>GLESFSLTSHEKKFGVNIEFSDVNFSYPKQTNHRTLKSINFFIPSGTTCALVGHTGSGKSTIAKLLYRFYDAEGDIKIGGKNVNKYNRNSIRSIIGIVPQDTILFNETIKYNILYGKL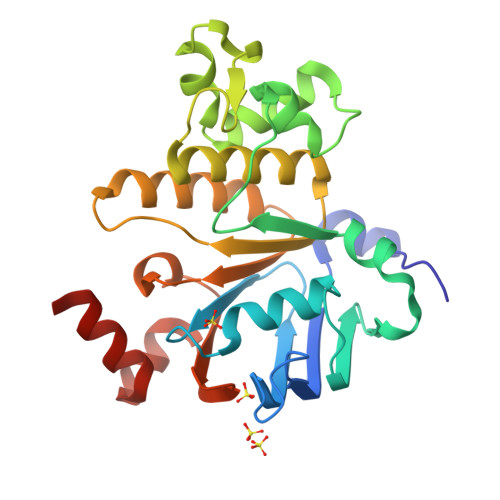DATDEEVIKATKSAQLYDFIEALPKKWDTIVGNKGMKLSGGERQRIAIARCLLKDPKIVIFDEATSSLDSKTEYLFQKAVEDLRKNRTLIIIAHRLSTISSAESIILLNKGKIVEKGTHKDLLKLNGEYAEMWNMQSGGNDI[4x]> ADDIVLKAKNGDVKFPHKAHQKAVPDCKKCHEKGPGKIEGFGKEMAHGKGCKGCHEEKKKGP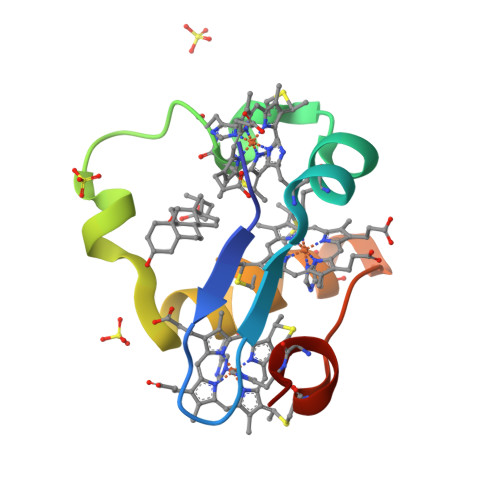TKCGECHKK Cell-traversal protein for ookinetes and sporozoites (CelTOS) is unique among traversal proteins as it is essential for traversal of malaria parasites in both the mosquito vector and human host and is therefore critical for malaria transmission and disease pathogenesis. Even though CelTOS is critical during cell traversal by malaria parasites and is a leading transmission- and infection-blocking malaria vaccine candidate, its function remains unknown as it has no sequence similarity to proteins of known function. We show that CelTOS specifically binds phosphatidic acid, a lipid predominantly found in the inner leaflet of plasma membranes, and potently disrupts defined liposomes composed of phosphatidic acid. Additionally, microinjection of CelTOS into Xenopus oocytes results in membrane damage. Together, these results demonstrate CelTOS is the only known apicomplexan protein with universal inner leaflet cellular activity as it addresses phosphatidic acid found specifically on the cytoplasmic face of plasma membranes, and disrupts these membranes to enable the exit of apicomplexan parasites through diverse vector and host cells.

The mechanism by which CelTOS enables the traversal of apicomplexan parasites through cells within the mammalian host and arthropod vector has been elusive because CelTOS has no sequence similarity to proteins of known function. Therefore, we determined the crystal structure of CelTOS from the human pathogen P. vivax (PvCelTOS) in order to obtain insight into function (Figure 1—figure supplement 2 and Figure 1—source data 1). CelTOS forms an alpha helical dimer that resembles a tuning fork. The dimer has a large buried surface area of 3003 Å2. Consistent with the structure and large buried surface area, we established that CelTOS is an obligate dimer in solution by sedimentation equilibrium analytical ultracentrifugation (Figure 1—source data 2). Two N-terminal helices (α-helices 1 and 2) of one monomer pack against the C-terminal helices (α-helices 3 and 4) of a second monomer to form the dimer. The outer surface of the CelTOS dimer is mildly hydrophilic and masks inner hydrophobic surfaces created between the two tines of the CelTOS dimer and the dimer interface. Strikingly, CelTOS resembles class I viral membrane fusion glycoproteins and a bacterial pore-forming toxin with roles in membrane binding and disruption. The C-terminal helices of CelTOS show structural similarity to HIV-1 gp41 and Mycobacterium bovis ESAT-6, and the N-terminal helices show similarity to Hendravirus fusion core; Nipahvirus fusion subunit core. The dimeric nature of CelTOS may serve as a chaperone-like function to retain CelTOS in an inactive state prior to membrane binding as the dimer masks the inner hydrophobic faces of CelTOS.

>[3x]MGLRGKSGSTASSSLEGGSEFSERIGNSLSSFLSESASLEVIGNELADNIANEIVSSLQKDSASFLQSGFDVKTQLKATAKKVLVEALKAALEPTEKIVASTIKPPRVSEDAYFLLGPVVKTLFNKVEDVLHKPIPDTIWEYESKGSLEEEEAEDEFSDELLDLEHHHHHH> GAASEIEKRQEENRKDREKAAAKFREYFPNFVGEPKSKDILKLRLYEQQHGKCLYSGKEINLGRLNEKGYVEIDHALPFSRTWDDSFN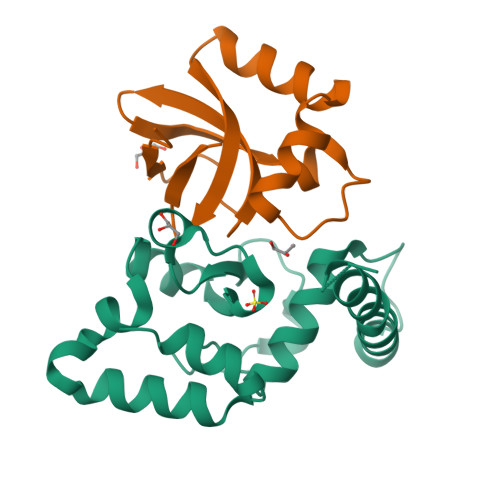NKVLVLGSENQNKGNQTPYEYFNGKDNSREWQEFKARVETSRFPRSKKQRILLQ;> MANKTYKIGKNAGYDGCGLCLAAISENEAIKVKYLRDICPDYDGDDKAEDWLRWGTDSRVKAAALEMEQYAYTSVGMASCWEFVEL Transmembrane channel-like (TMC) proteins are ion channels whose function has been linked to a variety of mechanosensitive processes, including hearing and balance in vertebrates and touch sensation in worms. The C. elegans genome encodes two tmc genes, tmc-1 and tmc-2, both of which encode proteins that are likely subunits of mechanosensitive ion channel complexes. By contrast, C. elegans TMC-2 is localized exclusively to body wall and vulval muscles and its role in worm physiology is less well explored. Here, we use cryo-electron microscopy (cryo-EM) to solve the structure of the native TMC-2 complex isolated from transgenic worms.

Particles that corresponded to a cis-dimeric complex were selected for subsequent refinement and 3D reconstruction, yielding a density map at 3.2 Å resolution, sufficient for model building. As in TMC-1, the TMC-2 complex harbors two copies each of TMC-2, CALM-1, and TMIE. Each TMC-2 protomer consists of 10 transmembrane helices and the dimer interface is composed of domain-swapped transmembrane helix 10 (TM10). The cytosolic domain includes six helices oriented nearly parallel to the membrane plane, all of which form extensive interactions with CALM-1. Unlike TMC-1, TMC-2 is not C2 symmetric owing to the orientation of the TM10 helices, which are offset by 10-16 Å relative to the TMC-1 TM10 helices. Density features consistent with glycosylation are observed at N225, located in the loop between TM1 and TM2, as well as N748, located in the loop between TM9 and TM10. A phospholipid occupies the cleft between TMC-2 H3 and TM1 (“cleft” lipid), and another resides in the cavity between the TMIE transmembrane helix and TMC-2 TM6 and TM8 (“bridge” lipid). An additional density feature that is consistent with a cholesterol molecule resides proximal to the extracellular side of TM2 in both structures. The pore appears closed and is blocked by three sites of constriction. We observed a second TMIE palmitoylation site on C43 in the TMC-2 complex structure that may have additional implications for gating of TMC ion channels.

>[2x]MPKSGAHQPLVRHDTDDGGETGQSVKSLADVSEEEIDSRMSRRSSVIADLLSLFRRSSSVLVRPHTRLGNPNFDDDDDEFDEEDDKEASKDRILKKIQQKKEIIQKLRGQPWYMKRKRRTLKVAQKHLQQQEAKVSKARLYKAEAGRRLTQASRWLDNLKIYLIPWEAKIRKIESHFGSVVSSYFTFHRWVLGVNITITFIMCMFVVIPEWLADSRTQFGDDRYNKTKAIKVMPPAVRARADELSTVWDFGGYFQYSLLFYGFYSKETFFGETIKYRVPVAYFFCNIFILGFSLFIILRKMAANNRRGTLSSGKTQQYLFNWKAFTGWDYTIGNPETAGNVYMANVIKFREAINDDKQKPSDKHPWIRFVARVLTNLFICAMYVFSIWAIMQCGTLKGEHFFAQNATAITISLITLVFPNIFDLLGKIEKLHPRNALRFQLGRVLVLYILNYYTLIYSLMLQLEHLQKEKNASDNPISALGHPGDAIGRTIRETVLPRYPVDNNPHTYYSYAPVTTTPIPATSSWTTVLPDFGPFGVYNPKASVTKDDTVFSSPVVETHMFGPNSDWNETTVNAASPTGATTRASLRMSQGGLCWETIIGQEITKLVTMDLYMTVASIFLIDFLRGLACRYLNLYWPWDLERTFPEYGEFKVAENVLHLVNNQGMIWLGLFFVPLLPMLNNIKLIILMYIRGWAAMTCNVPASQIFRASRSSNFFFALLILFLFLCTLPVGFVIASKTPSKSCGPFGNQSFFYSVITDVLHENLDKTLVNGIKYSLSPGIIIPVLVLLSLVIYFLIAMVTGLSQANQDLSFQLMVERTEEKKKIFELAGGKKKKSKDNTFGKQKPKQLLPPPTKGVSSDDDSQHNRSTAKSVSGRQFVPSLGSVSEVDHSTGEEQSSDSESTTSSLPPKLSLRQRFLVCIGWADPNKYGRHDDIEMEEGGGRLRELSTGSETDSDDEDSEKSNRDMSYRTAIQSFDQNSQSASASSSKSTTTAPSNSEMRIEITENPLHTYITPLRIEKKSSASSSSSSHQPSSSIEKQAARRLLQPISTTHNIRYGVATVENSSQDPTRPPSTDDSLGDPALHEPLWANLNPHSSYTSAMMSPIMNEVMSNDETTDDEKGRLIPDRPPIPHSPRELKRLKREKDQQSESGSKPSTPRPPRFRISMSPPRKPPSEKNDSDSSNRKYEMRVEKSPKKPKKSDND;>[2x]MGNNASSLSELNLFSKGGVFTREQLDEYQDCTFFTRKDIIRLYKRFYALNPHKVPTNMQGNRPAITTLTFEEVEKMPELKENPFKRRICEVFSEDGRGNLSFDDFLDMFSVFSEMAPLQLKLKYAFRIYDYDGDELLGHDDLSKMIRSLTRDELSDVEVEFIIERIIEEADLDGDSSINFAEFEHVVSRSPDFIRTFHIRI;>[2x]MPSGNEEINHLSALDQFVAPGLRLWMLIALVGGVLLIMIVIVCCFMRIRIPRTKRQIDLIAAKRKLRKSTKNSAEANAHNDERAQAIVMNSMPSGGGGGAPSTSSSRHTGSRIQSQV> MHDSPLKSLSAASNVASVNDPLFDFFNKHMGKQILIITESSQLNILGQTFRPIFCG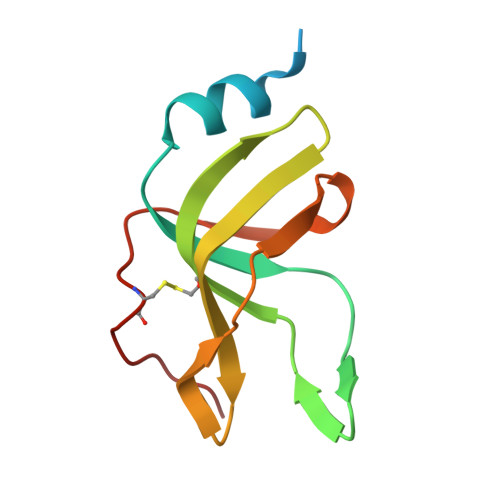KVAEVEPGHLTLSPVTIKILNAPFHKFPIPLSIPFEKIAHFTTDVDCSMRIPLV>MFNSDNLRLDGKCAIITGAGAGIGKEIAITFATAGASVVVSDINADAANHVVDEIQQLGGQAFACRCDITSEQELSALADFAISKLGKVDILVNNAGGGGPKPFDMPMADFRRAYELNVFSFFHLSQLVA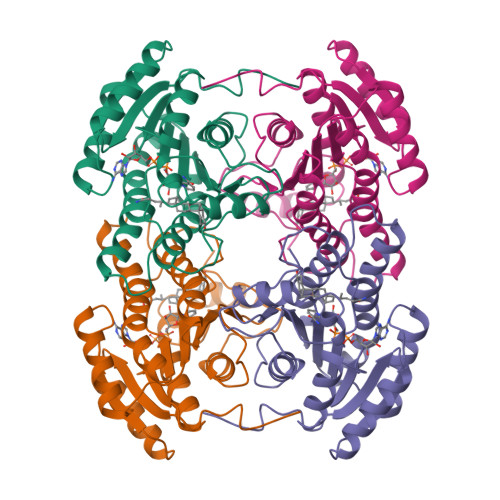PEMEKNGGGVILTITSMAAENKNINMTSYASSKAAASHLVRNMAFDLGEKNIRVNGIAPGAILTDALKSVITPEIEQKMLQHTPIRRLGQPQDIANAALFLCSPAASWVSGQILTVSGGGVQELN[2x]> SGPSGPATSDRSVVSESTVSWAAGARAVLRCQSPRMVWTQDRLHDRQRVVHWDLSGSKAGGPARRLVDMYSTGEQRVGEQRLGEQRVGEQRVYEPRDRGRLLLPPSAFHDGNFSLFIRAVEETDEGLYTCNLHHHYCHLYESLAVSLEVTDDPRAAGAHWDGEKEVLAVERGAPALLTCVNRAH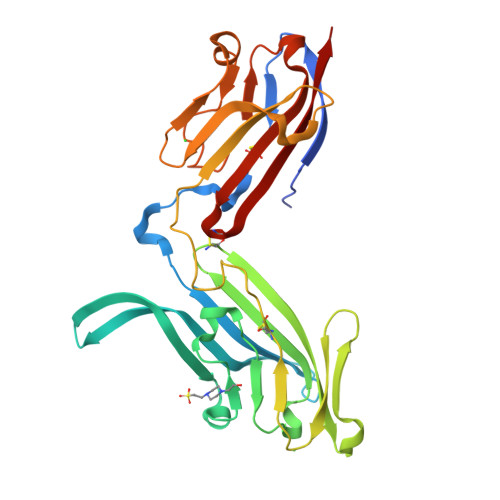VWTDRHLEEAQQVVHWDRQPPGVPHDRADRLLDLYASGERRAYGPPFLRDRVAVEADAFARGDFSLLIDPVEPADEGTYSCHLHHHYCGLHERRVFHLRVTE N-{3-[(4R,5R)-2-amino-5-fluoro-4-methyl-5,6-dihydro-4H-1,3-oxazin-4-yl]-4-fluorophenyl}-5-cyanopyridine-2-carboxamide 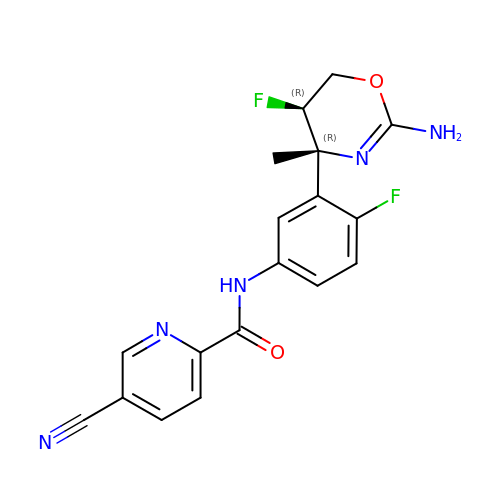| C18 H15 F2 N5 O2 | ALKHFUPBQSAGMS-MAUKXSAKSA-N> SSVPGFEKLANLLKPKPGLKKLLKWADAKKPPETVFTRLRLDKTGTQLFDNTDFPVWAAYTRSVAQTDSEASAVMLKTLVSRYSDEVLSGMIAAAKKSSKTESIATKLETEQMRTWLAAKKTPDDMFLVFKLNKAGDDILSSPLLSAWTNYMKLSNKENPKAQTTLIATMTKHYGDSGVSQILAAARKSPATQSTAKRLEAEQVQLWLKKGRTPDDTFTLLSLDRAGDDLLASPQFNTWMKYINYYNKENPDEKTTVLAKLMTHFDDEELTPILVVARKVPSTESTAAKLQAEQFKNWLSADKSPEEAFTLLQLDKAGDDLLTNPQLTNWLKYTENFNLNKEINEQVTAIQVFRAQYVDDSRIANMVIAAEKVPNTQAIAKRVEDELFKGWTVVLNKPDDVFINLKLETVGENVFESPLWSFYTKFLEKYNTANPGKEQTMISGLARGYNDVTLTNMLLKAKEAPSTKTLATKLEDELVQYWLADKKLPDKLFGYLELKESVDGILTNPVFNVWLKYLNAFNDKAPVKKALMIDTLKSAFGDVAVSNMLFAAKKDPGTAKVAATLQTA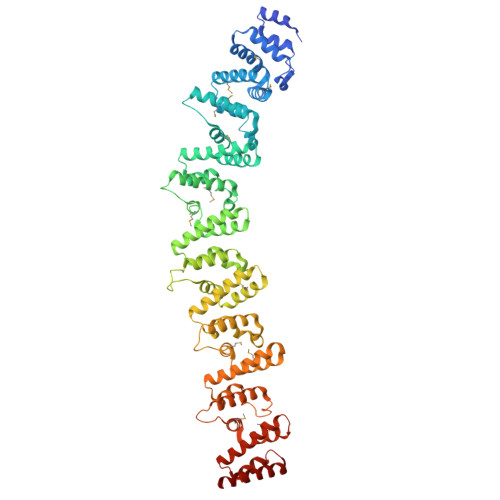LLSKWVLEKKTPGQVSAILKEGAGADVSAKLLATYSAKFKVRWG>GLGINEISSSFFSLLLEILLLESQ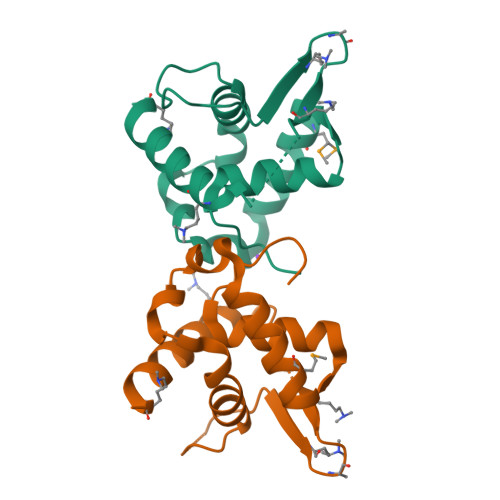ASLPMLEERVLDWQSSPASSLNSWFSAAPNWAELVLPALQYLAGESRAVPSSFSPFVEFKEKTQQWKLLGQSQDNEKELAALFQLWLETKDQAFCKQENEDSS[2x]> MNASEFRRRGKEMVDYVANYMEGIEGRQVYPDVEPGYLRPLIPAAAPQEPDTFEDIINDVEKIIMPGVTHWHSPYFFAYFPTASSYPAMLADMLCGAIGCIGFSWAASPACTELETVMMDWLGKMLELPKAFLNEKAGEGGGVIQGSASEATLVALLAARTKVIHRLQAASPELTQAAIMEKLVAYSSDQAHSSVERAGLIGGVKLKAIPSDGNFAMRASALQEALERDKAAGLIPFFMVATLGTTTCCSFDNLLEVGPICNKEDIWLHVDAAYAGSAFICPEFRHLLNGVEFADSFNFNPHKWLLVNFDCSAMWVKKRTDLTGAFRLDPTYLKHSHQDSGLITDYRHWQIPPGRRFRSLKMWFVFRMYGVKGLQAYIRKHVQLSHEFESLVRQDPRFEICVEVILGLVCFRLKGSNKVNEALLQRINSAKKIHLVPCHLRDKFVLRFAICSRTVESAHVQRAWEHIKELAADVLRAERE

Aromatic amino acid decarboxylase (AADC) deficiency is a severe inherited recessive neurotransmitter disorder caused by an impairment in dopamine synthesis due to the lack/modification of AADC, the enzyme converting l‐dopa to dopamine. Patients exhibit severe movement disorders and neurodevelopmental delay, with a high risk of premature mortality.

We then transfected the DDC‐KO cells with two AADC catalytic variants, R347Q and L353P, which resulted in loss‐of‐function and an altered profile of dopamine metabolites. By combining several structural approaches (X‐ray crystallography, molecular dynamics, small angle X‐ray scattering, dynamic light scattering, and spectroscopy), we determined that both variants alter the flexibility of the structural element to which they belong, whose integrity is essential for catalysis. This change causes a mispositioning of essential residues at the active site, leading, in turn, to an unproductive external aldimine, identifying the molecular basis for the loss‐of‐function.> MQTVNEMLRRAATRAPDHCALAVPARGLRLTHAELRARVEAVAARLHADGLRPQQRVAVVAPNSADVVIAILALHRLGAVPALLNPRLKSAELAELIKRGEMTAAVIAVGRQVADAIFQSGSGA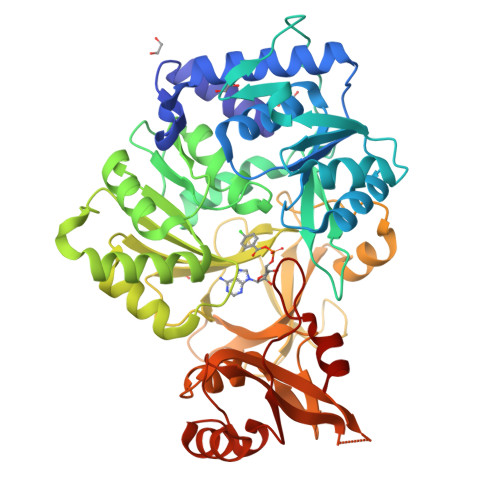RIIFLGDLVRDGEPYSYGPPIEDPQREPAQPAFIFYTSGTTGLPKAAIIPQRAAESRVLFMSTQVGLRHGRHNVVLGLMPLYHVVGFFAVLVAALALDGTYVVIEEFRPVDALQLVQQEQVTSLFATPTHLDALAAAAAHAGSSLKLDSLRHVTFAGATMPDAVLETVHQHLPGEKVNIYGTTEAMNSLYMRQPKTGTEMAPGFFSEVRIVRIGGGVDEIVANGEEGELIVAASDSAFVGYLNQPEATAEKLQDGWYRTSDVAVWTPEGTVRILGRVDDMIISGGENIHPSEIERVLGTAPGVTEVVVIGLADQRWGQSVTACVVPRLGETLSADALDTFCRSSELADFKRPKRYFILDQLPKNALNKVLRRQLVQQVSS>[18x]MANMEARNVM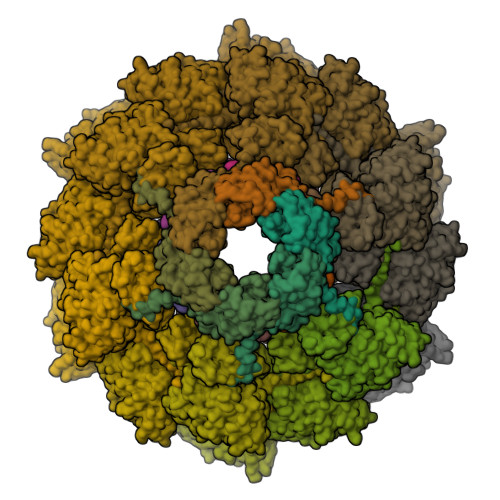SGTWGELWLDGNKVAEVKKFQAKMEFTKEDIIIAGQMGTDTKYMGYKGKGSITLYHVSSRMHKLIGEKIKRGSEPRFVAISKLNDPDSYGAERIAVKNIAFDDLTLADWEVGVKGEIEAPFTFTEYDFLDII;>MAIGLPSINISFKELATTVKERSARGIIAMVLKDAKALGLNEIHEKEDIPVDLSAENKEYINLALMGNVNTPNKLLVYVIEGEADIQTALDFLETKEFNYLCMPKAVEADKTAIKNWIIKLRDIDKVKVKAVLGKVVGNHEGIINFTTEDVLVGEKKYSVDEFTSRVAGLIAGTPLSQSVTYTKLSDVVDIPKMTKVDAESRVNKGELILIKEAGAIRIARGVNSLTELTAEKGEMFQKIKIVDTLDIIHSDIRKVIIDDYIGKVTNSYDNKCLLIVAIKSYLEELEKSALIESDSTVEIDFEAQKSYLKSKGVDLSYMTLQEIKEANTGSKVFLKAKIKVLDAMEDIDLSIEI[18x];>[6x]MLKYKEILETIIEILKKNFTESIFIDDESVQGSEGSCFFVSILSVICTPVMLNTNNKDIVISIKYLPKPQSKSIRMYEISDELNKLFNRNIKVTDRKLNITKLEQSIKKEESIYVLNFTFTLNYLDSVYEEDVVYENMKEINLNLGE> MSESGHSQPGLYGIERRRRWKEPGSGGPQNLSGPGGRERDYIAPWERERRDASEETSTSVMQKTPIILSKPPAERSKQPPPPTAPAAPPAPAPLEKPIVLMKPREEGKGPVAVTGASTPEGTAPPPPAAPAPPKGEKEGQRPTQPVYQIQNRGMGTAAPAAMDPVVGQAKLLPPERMKHSIKLVDDQMNWCDSAIEYLLDQTDVLVVGVLGLQGTGKSMVMSLLSANTPEEDQRTYVFRAQSAEMKERGGNQTSGIDFFITQERIVFLDTQPILSPSILDHLINNDRKLPPEYNLPHTYVEMQSLQIAAFLFTVCHVVIVVQDWFTDLSLYRFLQTAEMVKPSTPSPSHESSSSSGSDEGTEYYPHLVFLQNKARREDFCPRKLRQMHLMIDQLMAHSHLRYKGTLSMLQCNVFPGLPPDFL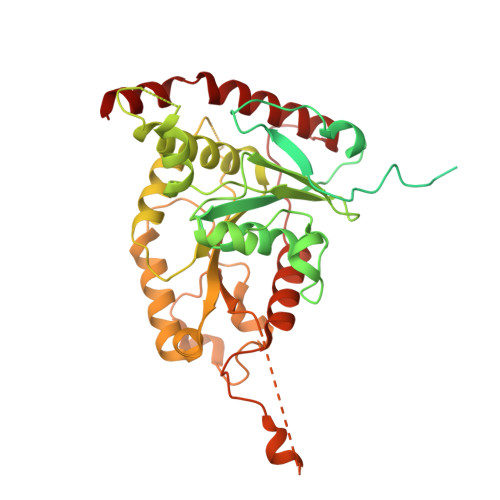DSEVNLFLVPFMDSEAESENPPRAGPGSSPLFSLLPGYRGHPSFQSLVSKLRSQVMSMARPQLSHTILTEKNWFHYAARIWDGVRKSSALAEYSRLLA>MEKLHQCYWKSGEPQSDDIEASRMKRAAAKHLIERYYHQLTEGCGNEACTNEFCASCPTFLRMDNNAAAIKALELYKINAKLCDPHPSKKGASSAYLENSKGAPNNSCSEIKMNKKGARIDFKDVTYLTEEKVYEILELCREREDYSPLIRVIGRVFSSAEALVQSFRKVKQHTKEELKSLQAKDEDKDEDEKEKAACSAAAMEEDSEASSSRIGDSSQGDNNLQKLGPDDVSVDIDAIRRVYTRLLSNEKIETAFLNALVYLSPNVECDLTYHNVYSRDPNYLNLFIIVMENRNLHSPEYLEMALPLFCKAMSKLPLAAQGKLIRLWSKYNADQIRRMMETFQQLITYKVISNEFNSRNLVNDDDAIVAASKCLKMVYYANVVGGEVDTNHNEEDDEEPIPESSELTLQELLGEERRNKKGPRVDPLETELGVKTLDCRKPLIPFEEFINEPLNEVLEMDKDYTFFKVETENKFSFMTCPFILNAVTKNLGLYYDNRIRMYSERRITVLYSLVQGQQLNPYLRLKVRRDHIIDDALVRLEMIAMENPADLKKQLYVEFEGEQGVDEGGVSKEFFQLVVEEIFNPDIGMFTYDESTKLFWFNPSSFETEGQFTLIGIVLGLAIYNNCILDVHFPMVVYRKLMGKKGTFRDLGDSHPVLYQSLKDLLEYEGNVEDDMMITFQISQTDLFGNPMMYDLKENGDKIPITNENRKEFVNLYSDYILNKSVEKQFKAFRRGFHMVTNESPLKYLFRPEEIELLICGSRNLDFQALEETTEYDGGYTRDSVLIREFWEIVHSFTDEQKRLFLQFTTGTDRAPVGGLGKLKMIIAKNGPDTERLPTSHTAFNVLLLPEYSSKEKLKERLLKAITYAKGFGML[2x];>[2x]MHQKRTAMFQDPQERPRKLPQLCTELQTTIHDIILECVYCKQQLLRREVYDFAFRDLCIVYRDGNPYAVCDKCLKFYSKISEYRHYSYSLYGTTLEQQYNKPLSDLLIRCINCQKPLSPEEKQRHLDKKQRFHNIRGRWTGRCMSCSRSSRTRRETQL

Human protein E6AP/UBE3A, the founding member of the HECT-type ubiquitin ligase family, was originally identified as an associated partner of the viral oncoprotein E6 of human papillomaviruses (HPVs). The E6 oncoprotein from high-risk HPV types hijacks the ligase activity of the host E6AP to ubiquitinate the tumor suppressor p5313, leading to the aberrant p53 degradation. The HECT-type E3 ligases have a characteristic C-terminal HECT domain consisting of an N-lobe and a C-lobe that are responsible for E2 binding and ubiquitin acceptance, respectively. Here, by using cryogenic electronic microscopy, we reveal that the structures of full-length E6AP and E6AP/E6 complex are monomer and dimer of E6AP/E6 protomer, respectively.

After several rounds of 3D classification, we identified five distinct conformational states of the E6AP/E6 complex and resolved the structures of these five conformations at resolutions ranging from 2.6 to 4.4 Å. We used the 2.6-Å density map to build the ab initio atomic model. The overall structure of the E6AP/E6 complex looks like two leaning “towers” standing on a base. Each tower derives exclusively from E6AP’s N-terminal region (residues 120-169, 231-384, and 427-483), whereas the base consists of the C-terminal HECT domain (residues 484–875), the loop-helix fragment, and the LxxLL-containing loop-helix-loop element (residues 385-426) stretching down from the tower region. We therefore assigned the five conformations into one of two classes: attached (Att) or detached (Det). In all three Att conformations, the catalytic C-lobe of E6AP attaches to E6, whereas, in the two Det conformations, there are no interactions between the C-lobe and E6. We hereafter refer to the three Att conformations as Att1, Att2 and Att3 based on the distance between the tips of the two towers in a descending sequence: 74 Å in Att1, 71 Å in Att2, and 66 Å in Att3. Only the zinc-binding E6N and E6C domains interact with the C-lobe of E6AP. Residues H31 and D32 of E6N form hydrogen bonds with T834 and R836 of the C-lobe, respectively. As the two towers underwent an outwards rotation, the Det2 conformation transformed into the Det1 conformation. Intriguingly, despite substantial variation in the structure of the E6AP/E6 complex, the inter–α1-helical interaction remains intact; albeit there are some changes at the interface between the two α1-helices (238 Å2 for Att1, 222 Å2 for Att2, 209 Å2 for Att3, 157 Å2 for Det1 and 145 Å2 for Det2).>[6x]MTDTHTGPTPADAVPAYPFSLPHALDLDPHYAELRRDEPVSRVRLPYGEGTAWLVTRMSDARIVLGDSRFSTAAATDPATPRMFPTPPEPDGVLAQDPPDHTRLRRLVGKAFTARRVEEMRPRVRSLVDSLLDDMVAHGSPADLVEFLAVPFPVAVICELLGVPLEDRDLFRTFSDAMLSSTRLTAAEIQRVQQDFMVYMDGLVAQRRDAPTEDLLGALALATDNDDHLTKGEIVNMGVSLLIAGHETSVNQITNLVHLLLTERKRYESLVADPALVPAAVEEMLRYTPLVSAGSFVRVATEDVELSTVTVRAGEPCVVHFASANRDEEVFDHADELDFHRERNPHIAFGHGAHHCIGAQLGRLELQEALSALVRRFPTLDLAEPVAGLKWKQGMLIRGLERQIVSW

The bacterial P450 OleP, from Streptomyces antibioticus, is an epoxidase involved in the tailoring steps of the biosynthetic pathway of the antibiotic oleandomycin. More specifically, OleP catalyzes a regio- and stereospecific reaction of epoxidation at the C8-C8a of the macrolactone ring. Among the known macrolide epoxygenases from actinomycetes, OleP presents a unique epoxidation chemistry since it targets a non-activated C-C bond, which is a reaction not easily achievable through conventional chemical synthesis protocols. In addition, discordant findings have been reported concerning the timing of OleP activity during the tailoring phase of oleandomycin biosynthesis, showing that OleP is either active on the aglycone intermediate, 8.8a-deoxyoleandolide (DEO), or on the monoglycosylated one, L-olivosyl-8.8a-deoxyoleandolide (L-O-DEO).

As observed for OleP-6DEBHS, high ionic strength conditions (I = 4 M) induced the crystallization of six copies of the closed OleP–DEO complex in the asymmetric unit. Higher ionic strength (I = 4 M) shifts the equilibrium towards the closed state in crystallo. In the closed state, the substrate displaces the sixth axial water ligand, with the macrolactone ring adopting the correct orientation where the C8-C8a bond is parallel and exposed to the heme plane, at a distance of about 4–5 Å from the iron, which is compatible with an initial attack of C8-C8a by activated oxygen species formed at the heme iron. In this position, DEO induces the formation of the helix I cleft, showing the conserved catalytical T248 lining a water channel that might enable proton delivery during OleP catalysis. A critical contribution to the correct positioning of DEO is provided by carbonyl–aromatic interactions that involve the carbonyl at C1 sandwiched between F296 on β-hairpin β3 and F84 on the BC loop. Only higher ionic strength conditions enable a unique positioning of DEO in the active site. In the latter conditions, a network of hydrogen bonds that forms between the C3-OH and the C5-OH of DEO and solvent molecules trapped in the small cavity, the solvent cavity, of the active site, constrains the substrate position and bridges its contacts with the enzyme on regions directly involved in the open-to-closed transition. Although not determinant for triggering the closure, these water/formate-mediated interactions contribute to the stabilization of the closed state. In this analysis, L-O-DEO was docked into the active site of the closed OleP–DEOHS structure using Autodock Vina 1.1.2.>[2x]KDIKKQITDINYLLLKNEEYKKYDIKKYNFFSSGKKINKGNIHLLTKQMRTFKEIFFSLGFEEMETHNYVESSFWCFDALYIPQQHPSRDLQDTFFIKEPETCIDKFVDTEYIDNIKRVHTHGDYGSFGWNYKWKLEESKKNVLRTHTTAN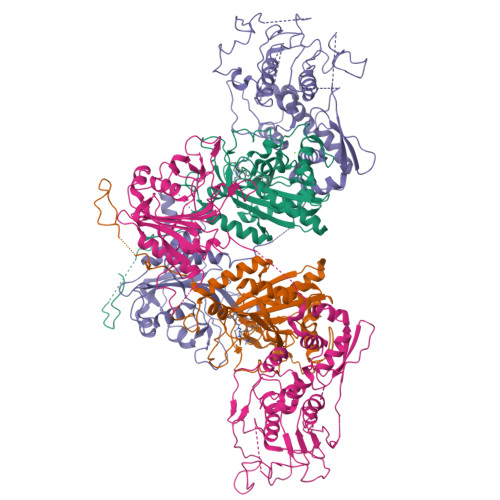SCRALFKLAKEYKEAGCIKPKKYFSIDRVFRNENLDSTHLAEFHQVEGLIIDKNIGLSHLIGTLAAFYKHIGIHKLKFKPTFNPYTEPSMEIYGYHEQSKKWLEVGNSGIFRPEMLRSMGFSEEVSVIAWGLSLERPTMIKYNIKNIRDLFGYKSVV;>MPTISVYEDDLFEKLGEEIIEEKLLDVCFDFGLEVDDIEYKNDKKIYKIEVPANRYDLICVEGLCRALKNFMCKFDDIKYDISMNNYDICIKGNQYIKVDGSVDDRRGYVVCCVLKNMNINDSVYNNIIEIQEKLHHNLGKKRSVLAIGIHDYDKIKFPLKYKFEKKEKINFIPLNEKTNLNGMNLIDFYSKNLNLKPYLKIIKDFDKYPIIVDSNEQILSLPPIINCDHTKISLNTKNVFIECTAIDRNKAQIALNILCSMLSEYCVPKYSIQSFVVIYENQDFSDDQNLKKKETQFLYPIFENKSLTCNIDYVRKLSGISHITVHEVNNLLKRMMLSCDIMDNNTFKVTIPFYRSDIMHCCDIIEDIAIAYGYGNIKYEPPQICKKHSLNNCSELFRNVLVECGYTEVMTNALLSRDENYNCMLRTHKSYDDPNINLDEYNPLAAPIQIKNSKTSEYEIIRTSLIVNLLKFVSANKHRELPLRFFEIGDVSYATYNQTDTNAVNKKYLSIIFSDKFTAGLEELHGVLEAILKEYQLFSDYKIEEKKKENISIRSDMYYKLIPKEDPSFLNERIVDIVLFPHNLKFGVLGIIHPKVLENFSLDIPVSAIEINVETLLNVLMM[2x]> MTTSVFVSGATGYLAQQIIALVLSKGYKVVGSVRSEEKGANLKKLYGDDFSYEVVKVLEQKGAFD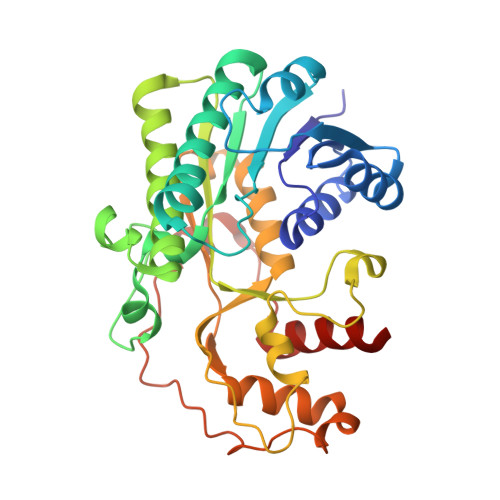EALKKHPEVTIFLHTASPVTFEVEDTEKEILIPAINGTKYVLQSIKDVAPQITRVVYTSSVVAMSVPEELGSPDVVLSEASWSSLSYEQSKTHGVLAYFGSKQFAERAAWEFVEQEKPNFALSTVNPVYIFGPQAKDEEVKGTLNHSAEMVNSVLKLNKDDDVPATTGTFIDVRDVAKAHLAAFEKDEAKGERLLLSNTRFNGQTLLDVVRKNFPQLADKLPVGKPHSDDFSAFKEWNDKKTKKILGFEYFDFETSVVDSIKQVLKVQG>[2x]MKKIEVYAQPDCPPCVIVKEFLKHNNVAYEEFDVKKDAAARNR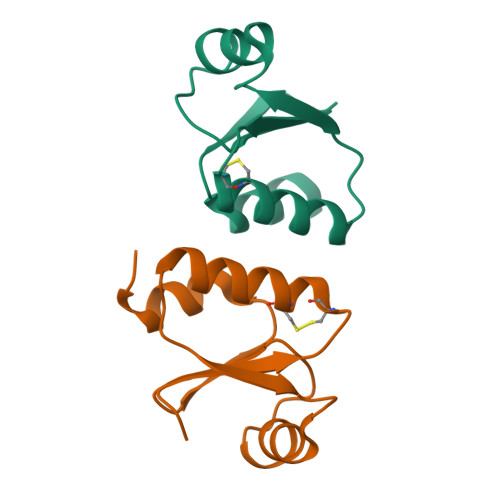LLYDYDSYSTPTVVIDGEVVAGFQIEKLQQLLNIE4,4'-{3-[(4-hydroxyphenyl)amino]-1H-pyrazole-4,5-diyl}diphenol | C21 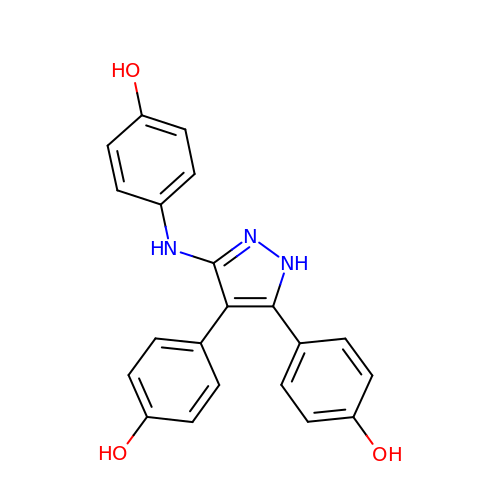H17 N3 O3 | VIJBEUTVNBPGIU-UHFFFAOYSA-N> PEFMVTTEPALADLQEQLYNGNEKSQLAAMSTLSTAGTEGYHLLQEFLKDSATFSPPPAPWIRGQAYRLLFHSPEASVQAFLQQHYPQGVIPLRSDRGVDYQELAKLFVAEKFEAADRLTTQKLCELAGPLAQKRRWLYFTEVEQLPIPDLQTIDQLWLAF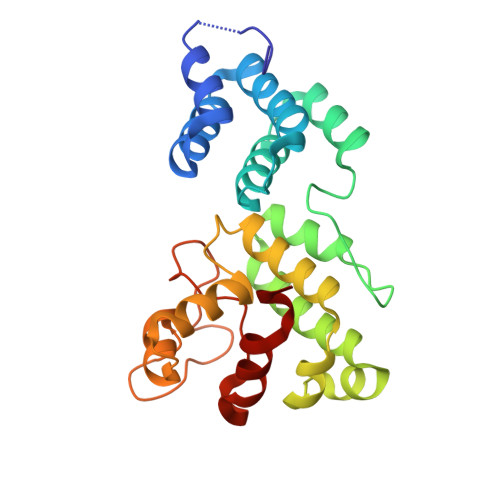SLGRFGYSVQRQLWLGCGQNWDRLWEKIGWRQGKRWPRYPNEFIWDLSAPRGHLPLTNQLRGVQVLNALLNHPAWTA The protein GtgE has been identified as a cysteine protease that targets members of the Rab-family. Rab32 is involved in controlling the biogenesis of lysosome-related organelles (LRO). It is believed that GtgE inactivates Rab32 proteolytically and thereby prevents the delivery of antimicrobial factors that would impair Salmonella infection. Furthermore, by using a combination of biochemical characterization, molecular dynamics simulation, and binding studies, we demonstrate that GtgE shows exclusive selectivity for the inactive GDP-bound state of Rab32.

Crystals obtained after reductively alkylating the truncated Rab3218-201:GDP:GtgE21-214,C45A-complex and the full-length complex Rab321-225:GDP:GtgE1-228,C45A diffracted up to 2.3 Å and 2.9 Å resolution, respectively. The average B-factor of the full-length complex is higher than for the truncated complex, though the entire electron density is well defined for both structures. Due to the higher resolution, the truncated Rab3218-201:GDP:GtgE21-214,C45A-complex is discussed only and referred to as Rab32:GDP:GtgEC45A hereafter. In the complex structure, GtgE can be envisioned as a trident poking into Rab32 with three spike-like protrusions. Spike 2 is represented by the β2G–β3G loop (where subscript G denotes GtgE), and penetrates deeply into the switch I–switch II cleft of Rab32. Thereby, spike 1 and 2 form intimate interactions with the switch I structure that is also the site of proteolytic cleavage. The shallow cleft between spike 2 and 3 is filled by the switch II region of Rab32. In particular, the N-terminus (amino acids 23–45), including the position of the active sitecysteine (here the C45A substitution) is now resolved, in addition to the loop regions β2G-β3G (i.e., spike 2) and α4G-β6G (i.e., spike 3). The complex interface buries an average solvent exposed surface area of 1535 Å2, as determined with the ‘Protein interfaces, surfaces and assemblies’ web service (PISA). The switch I residue I58R forms the center of a hydrophobic cluster and interacts with W46G, L81G, C86G, I141G, L150G, and I202G, whereas D61R from the protease recognition sequence forms a specific interaction with the guanidinium group of R142G. The interacting polar network between the catalytic triad, C45G, H151G, and D169G, is formed in the Rab32:GDP:GtgEC45A-complex once C45G is modeled to the active site cysteine nucleophile.

> GHMQGQIIHHRNFQSQFDTTGNTLYNNAWVCSLNVIKSRDGNNYSALEDITSDNQAFNNILEGIDIIECENLLKEMNVQKIPESSLFTNIKEALQAEVFNSTVEDDFESFISYELQNHGPLMLIRPSLGSECLHAECIVGYDSEVKKVLIYDSMNTSPEWQSNIDVYDKLTLAFNDKYKNEDCSICGLYYDGVYEPK;> METREHLFKVLVIGELGVGKTSIIKRYVHQLFSQHYRATIGVDFALKVLNWDSRTLVRLQLWDIAGQERFGNMTRVYYKEAVGAFVVFDISRSSTFEAVLKWKSDLDSKVHLPNGSPIPAVLLANKCDKNKDSSQSPSQVDQFDKEHGFAGWFETSAKDNINIEEAARFLVEKILVNHQSFPN> AKALIVYGSTTGNTEYTAETIARELADAGYEVDCRDAASVEAGGLFEGFDLVLLGCSTWGDDSIELQDDFIPLFDSLEETGAQGRKVACFGCGDSSYEYFCGAVDAIEEKLKNLGAEIVQDGLRIDGDPRAARDDIVGWAH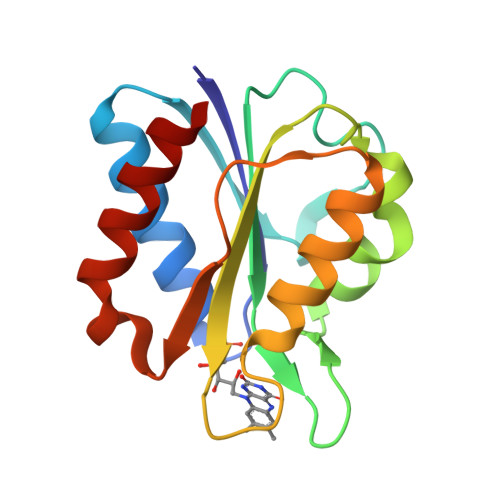DVRGAI>[2x]GSTWRQNTKSSRIEAIKIQILSKLRLETAPNISKDVIRQLLPKAPPLRELIDQYDVQRDDSSDGSLEDDDYHATTETIITMPTESDFLMQVDGKPKCCFFKFSSKIQYNKVVKAQLWIYLRPVETPTTVFVQILRLIKPMKDGTRYTGIRSLKLDMNPGTGIWQSIDVKTVLQNWLKQPESNLGIEIKALDENGHDLAVTFPGPGEDGLNPFLEVKVTDTPKRSRRDFGLDCDEHSTESRC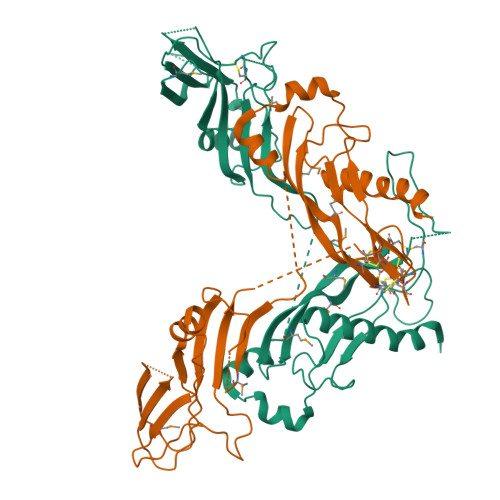CRYPLTVDFEAFGWDWIIAPKRYKANYCSGECEFVFLQKYPHTHLVHQANPRGSAGPCCTPTKMSPINMLYFNGKEQIIYGKIPAMVVDRCGCS> MSAYATQGFNLDDRGRRIVVDPVTRIEGHMRCEVNVDANNVIRNAVSTGTMWRGLEVILKGRDPRDAWAFVERICGVCTGCHALASVRAVENALDIRIPKNAHLIREIMAKTLQVHDHAVHFYHLHALDWVDVMSALKADPKRTSELQQLVSPAHPLSSAGYFRDIQNRLKRFVESGQLGPFMNGYWGSKAYVLPPEANLMAVTHYLEALDLQKEWVKIHTIFGGKNPHPNYLVGGVPCAINLDGIGAASAPVNMERLSFVKARIDEIIEFNKNVYVPDVLAIGTLYKQAGWLYGGGLAATNVLDYGEYPNVAYNKSTDQLPGGAILNGNWDEVFPVDPRDSQQVQEFVSHSWYKYADESVGLHPWDGVTEPNYVLGANTKGTRTRIEQIDESAKYSWIKSPRWRGHAMEVGPLSRYILAYAHARSGNKYAERPKEQLEYSAQMINSAIPKALGLPETQYTLKQLLPSTIGRTLARALESQYCGEMMHSDWHDLVANIRAGDTATANVDKWDPATWPLQAKGVGTVAAPRGALGHWIRIKDGRIENYQCVVPTTWNGSPRDYKGQIGAFEASLMNTPMVNPEQPVEILRTLHSFDPCLACSTH;> METKPRTPVLWLHGLECTGCSESFIRSAHPLAKDVVLSMISLDYDDTLMAAAGHQAEAILEEIMTKYKGNYILAVEGNPPLNQDGMSCIIGGRPFIEQLKYVAKDAKAIISWGSCASWGCVQAAKPNPTQATPVHKVITDKPIIKVPGCPPIAEVMTGVITYMLTFDRIPELDRQGRPKMFYSQRIHDKCYRRPHFDAGQFVEEWDDESARKGFCLYKMGCKGPTTYNACSTTRWNEGTSFPIQSGHGCIGCSEDGFWDKGSFYDRLTGISQFGVEANADKIGGTASVVVGAAVTAHAAASAIKRASKKNETSGSEHRSAWSHPQFEK

A prominent member of these so-called Knallgas bacteria is Cupriavidus necator H16 (formerly Ralstonia eutropha H16), which employs four different O2-tolerant [NiFe]-hydrogenases for generating cellular energy from the controlled oxidation of H2 in the presence of O2.5 Among them, only the tripartite membrane-bound [NiFe]-hydrogenase (MBH) is directly linked to the respiratory chain. The MBH large subunit contains the catalytic center composed of a nickel and an iron ion, which are coordinated to the protein by four Cys-derived thiolates. The most distal cluster relative to the active site is a [4Fe–4S] cluster coordinated by three cysteines and a histidine, while the medial cluster is a [3Fe–4S] species with three cysteines as protein anchors. However, in the proximal position, instead of a standard Cys4[4Fe–4S] cluster, the O2-tolerant MBHs possess a [4Fe–3S] cluster coordinated by six cysteine residues (Fig. 1 and S1†).13–16 The unique architecture of the [4Fe–3S] cluster is associated with a redox-dependent structural flexibility that allows two redox-transitions within a physiological potential region, i.e., the cofactor can assume a super-oxidized, an oxidized, and a reduced state. In order to obtain insight into the individual role of the supernumerary cysteines in the coordination and function of the [4Fe–3S] cluster, we purified C. necator MBH derivatives carrying exchanges of cysteine for glycine at the positions 19 and/or 120 in the small subunit HoxK, which are hereafter referred to as MBHC19G, MBHC120G and MBHC19G/C120G.

H2-reduced MBHC19G crystals harbored an almost cubic [4Fe–4S] cluster in the proximal position. In contrast to the native [4Fe–3S] cluster, the bridging function of the Cys19-derived thiolate was replaced with a sulfide (S4) coordinating both Fe1 and Fe4. Surprisingly, the Fe3 coordination to Cys120 was essentially lost. According to the electron density maps (Fig. S2†) only ca. 20% of Fe3 remained in the native-like (“classical”) position, previously observed for the Fe3 in the native [4Fe–3S] cluster. Approximately 80% of Fe3 were shifted by 1.4 Å to a position corresponding to a cubane corner (Fe3′), thereby forming a bond to S4 instead of Cys120. In H2-reduced MBHC19G crystals, a major fraction of Fe3 is not covalently bound to Sγ-Cys120, which is in contrast to the reduced [4Fe–3S] cluster of native MBH. This result can be explained by the fact that sulfide (S4) is a more tightly bound ligand than a thiolate, which leads to coordinative bonding to the shifted Fe3′. We interpreted this density as a mono-oxygen species with an occupancy of about 50%, causing a slightly enlarged Ni–Fe distance of 2.7 Å.2-[3-(tetrahydro-2H-pyran-4-yloxy)propyl]-1,2,3,4-tetrahydroisoquinolin-5-amine 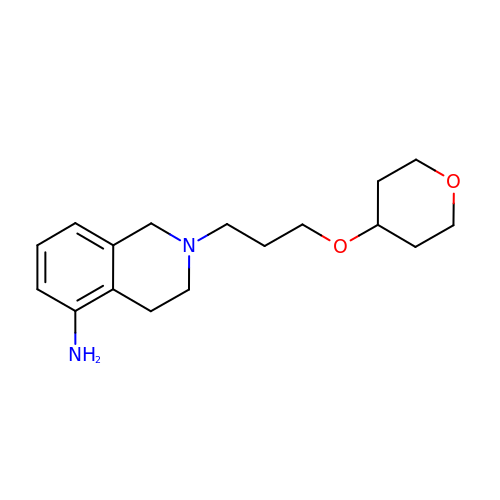| C17 H26 N2 O2 | LJEGYFBKFOMGEW-UHFFFAOYSA-N> SGSSLQQHLSNRDPRP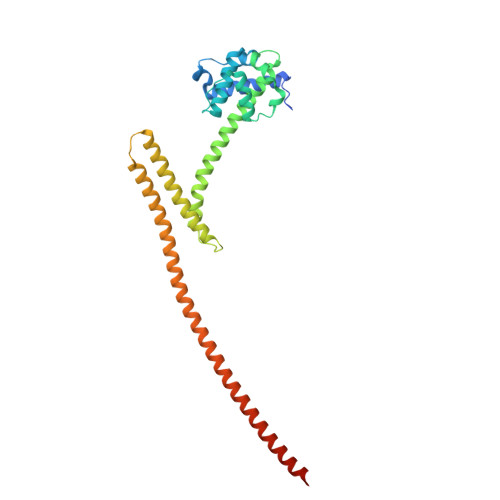LRDKNFQSAIQEEIYDYLKKNKFDIETNHPISIKFLKQPTQKGFIIIFKWLYLRLDPGYGFTKSIENEIYQILKNLRYPFLESINKSQISAVGGSNWHKFLGMLHWMVRTNIKLDMCLNKVDRSLINQNTQEITILSQPLKTLDEQDQRQERYELMVEKLLIDYFTESYKSFLKLEDNYEPSMQELKLGFEKFVHIINTDVTSTELKLEELKVDLNRKRYKLHQQVIHVIDITSKFKINIQSSLENSENELGNVIEELRNLEFETEHNVTN> MGAQVSTQKTGAHENQNVAANGSTINYTTINYYKDSASNSATRQDLSQDPSKFTEPV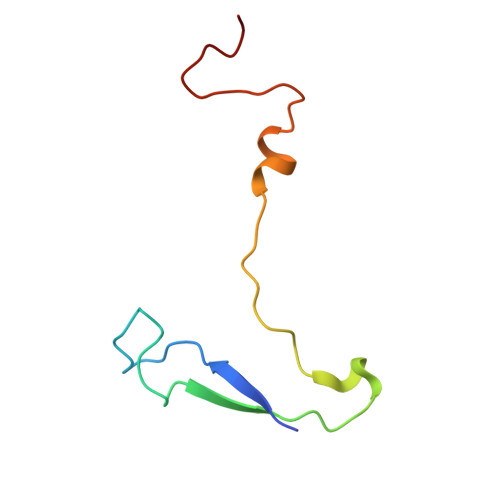KDLMLKTAPALN>MFEARLVQGSILKKVLEALKDLINEACWDISSSGVNLQSMDSSHVSLVQLTLRSEGFDTYRCDRNLAMGVNLTSMSKILKCAGNEDIITLRAEDNADTLALVFEAPNQEKVSDYEMKLMDLDVEQLGIPEQEYSCVVKMPSGEFARICRDLSHIGDAVVISCAKDGVKFSASGELGNGNIKLSQTSNVDKEEEAVTIEMNEPVQLTFALRYLNFFTKATPLSSTVTLIMSADVPLVVEYKIADMGHLKYYLAPKIEDEEGS[3x];>[3x]CGRKRRQTSM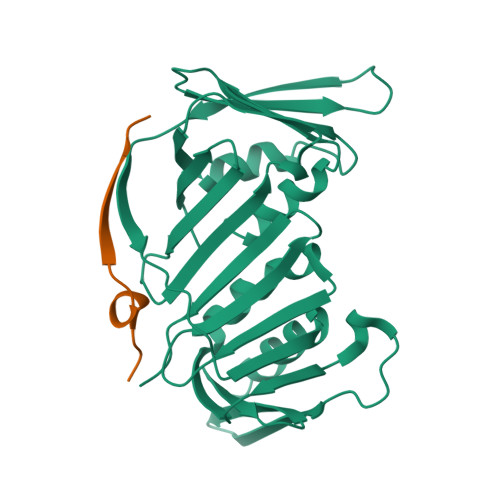TDFYHSKRRLIFS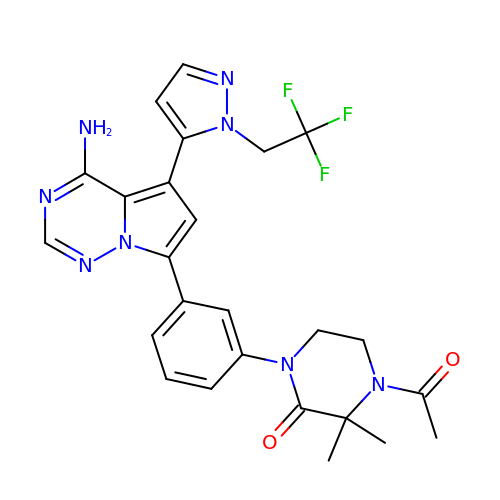4-acetyl-1-(3-{4-amino-5-[1-(2,2,2-trifluoroethyl)-1H-pyrazol-5-yl]pyrrolo[2,1-f][1,2,4]triazin-7-yl}phenyl)-3,3-dimethylpiperazin-2-one | C25 H25 F3 N8 O2 | KSAKMNJFOKNIAA-UHFFFAOYSA-N> ETGVFQKAVDQSIEKKIVLRNGTEAFDSWEKPPLPVYTQFYFFNVTNPEEILRGETPRVEEVGPYTYRELRNKANIQFGDNGTTISAVSNKAYVFERDQSVGDPKIDLIRTLNIPVLTVIEWSQVHFLREIIEAMLKAYQQKLFVTHTVDELLW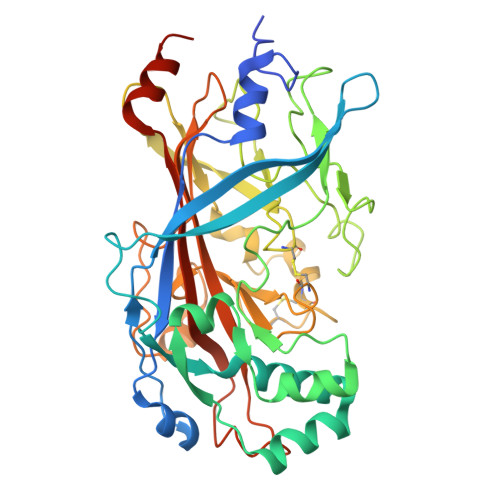GYKDEILSLIHVFRPDISPYFGLFYEKNGTNDGDYVFLTGEDSYLNFTKIVEWNGKTSLDWWITDKCNMINGTDGDSFHPLITKDEVLYVFPSDFCRSVYITFSDYESVQGLPAFRYKVPAEILANTSDNAGFCIPEGNCLGSGVLNVSICKNGAPIIMSFPHFYQADERFVSAIEGMHPNQEDHETFVDINPLTGIILKAAKRFQINIYVKKLDDFVETGDIRTMVFPVMYLNESVHIDKETASRLKSMINTTGKHHHHHH>MLDSKLKAPVFTVRTQGREYGEFVLEPLERGFGVTLGNPLRRILLSSIPGTAVTSVYIEDVLHEFSTIPGVKEDVVEIILNLKELVVRFLNPSLQTVTLLLKAEGPKEVKARDFLPVADVEIMNPDLHIATLEEGGRLNMEVRVDRGVGYVPAEKHGIKDRINAIPVDAVFSPVRRVAFQVEDTRLGQRTDLDKLTLRIWTDGSVTPLEALNQAVEILREHLTYFSNPQAAAVAAPEEAKEPEAPPEQEEELDLPLEELGLSTRVLHSLKEEGIESVRALLALNLKDLKNIPGIGERSLEEIKEALEKKGFTLKE[2x];> MEIKRFGRIREVIPLPPLTEIQVESYRRALQADVPPEKRENVGIQAAFRETFPIEEEDKGKGGLVLDFLEYRLGEPPFPQDECREKDLTYQAPLYARLQLIHKDTGLIKEDEVFLGHIPLMTEDGSFIINGADRVIVSQIHRSPGVYFTPDPARPGRYIASIIPLPKRGPWIDLEVEPNGVVSMKVNKRKFPLVLLLRVLGYDQETLARELGAYGELVQGLMDESVFAMRPEEALIRLFTLLRPGDPPKRDKAVAYVYGLIADPRRYDLGEAGRYKAEEKLGIRLSGRTLARFEDGEFKDEVFLPTLRYLFALTAGVPGHEVDDIDHLGNRRIRTVGELMTDQFRVGLARLARGVRERMLMGSEDSLTPAKLVNSRPLEAAIREFFSRSQLSQFKDETNPLSSLRHKRRISALGPGGLTRERAGFDVRDVHRTHYGRICPVETPEGANIGLITSLAAYARVDELGFIRTPYRRVVGGVVTDEVVYMTATEEDRYTIAQANTPLEGNRIAAERVVARRKGEPVIVSPEEVEFMDVSPKQVFSVNTNLIPFLEHDDANRALMGSNMQTQAVPLIRAQAPVVMTGLEERVVRDSLAALYAEEDGEVAKVDGNRIVVRYEDGRLVEYPLRRFYRSNQGTALDQRPRVVVGQRVRKGDLLADGPASENGFLALGQNVLVAIMPFDGYNFEDAIVISEELLKRDFYTSIHIERYEIEARDTKLGPERITRDIPHLSEAALRDLDEEGVVRIGAEVKPGDILVGRTSFKGESEPTPEERLLRSIFGEKARDVKDTSLRVPPGEGGIVVRTVRLRRGDPGVELKPGVREVVRVYVAQKRKLQVGDKLANRHGNKGVVAKILPVEDMPHLPDGTPVDVILNPLGVPSRMNLGQILETHLGLAGYFLGQRYISPIFDGAKEPEIKELLAQAFEVYFGKRKGEGFGVDKREVEVLRRAEKLGLVTPGKTPEEQLKELFLQGKVVLYDGRTGEPIEGPIVVGQMFIMKLYHMVEDKMHARSTGPYSLITQQPLGGKAQFGGQRFGEMEVWALEAYGAAHTLQEMLTLKSDDIEGRNAAYEAIIKGEDVPEPSVPESFRVLVKELQALALDVQTLDEKDNPVDIFEGLASKR;> MKKEVRKVRIALASPEKIRSWSYGEVEKPETINYRTLKPERDGLFDERIFGPIKDYECACGKYKRQRFEGKVCERCGVEVTKSIVRRYRMGHIELATPAAHIWFVKDVPSKIGTLLDLSATELEQVLYFSKYIVLDPKGAILNGVPVEKRQLLTDEEYRELRYGKQETYPLPPGVDALVKDGEEVVKGQELAPGVVSRLDGVALYRFPRRVRVEYVKKERAGLRLPLAAWVEKEAYKPGEILAELPEPYLFRAEEEGVVELKELEEGAFLVLRREDEPVATYFLPVGMTPLVVHGEIVEKGQPLAEAKGLLRMPRQVRAAQVEAEEEGETVYLTLFLEWTEPKDYRVQPHMNVVVPEGARVEAGDKIVAAIDPEEEVIAEAEGVVHLHEPASILVVKARVYPFEDDVEVSTGDRVAPGDVLADGGKVKSDVYGRVEVDLVRNVVRVVESYDIDARMGAEAIQQLLKELDLEALEKELLEEMKHPSRARRAKARKRLEVVRAFLDSGNRPEWMILEAVPVLPPDLRPMVQVDGGRFATSDLNDLYRRLINRNNRLKKLLAQGAPEIIIRNEKRMLQEAVDALLDNGRRGAPVTNPGSDRPLRSLTDILSGKQGRFRQNLLGKRVDYSGRSVIVVGPQLKLHQCGLPKRMALELFKPFLLKKMEEKGIAPNVKAARRMLERQRDIKDEVWDALEEVIHGKVVLLNRAPTLHRLGIQAFQPVLVEGQSIQLHPLVCEAFNADFDGDQMAVHVPLSSFAQAEARIQMLSAHNLLSPASGEPLAKPSRDIILGLYYITQVRKEKKGAGLEFATPEEALAAHERGEVALNAPIKVAGRETSVGRLKYVFANPDEALLAVAHGIVDLQDVVTVRYMGKRLETSPGRILFARIVAEAVEDEKVAWELIQLDVPQEKNSLKDLVYQAFLRLGMEKTARLLDALKYYGFTFSTTSGITIGIDDAVIPEEKKQYLEEADRKLLQIEQAYEMGFLTDRERYDQILQLWTETTEKVTQAVFKNFEENYPFNPLYVMAQSGARGNPQQIRQLCGLRGLMQKPSGETFEVPVRSSFREGLTVLEYFISSHGARKGGADTALRTADSGYLTRKLVDVTHEIVVREADCGTTNYISVPLFQPDEVTRSLRLRKRADIEAGLYGRVLAREVEVLGVRLEEGRYLSMDDVHLLIKAAEAGEIQEVPVRSPLTCQTRYGVCQKCYGYDLSMARPVSIGEAVGIVAAQSIGEPGTQLTMRTFHTGGVAGAADITQGLPRVIELFEARRPKAKAVISEIDGVVRIEETEEKLSVFVESEGFSKEYKLPKEARLLVKDGDYVEAGQPLTRGAIDPHQLLEAKGPEAVERYLVEEIQKVYRAQGVKLHDKHIEIVVRQMMKYVEVTDPGDSRLLEGQVLEKWDVEALNERLIAEGKTPVAWKPLLMGVTKSALSTKSWLSAASFQNTTHVLTEAAIAGKKDELIGLKENVILGRLIPAGTGSDFVRFTQVVDQKTLKAIEEARKEAVEAKERPAARRGVKREQPGKQA;> MAEPGIDKLFGMVDSKYRLTVVVAKRAQQLLRHGFKNTVLEPEERPKMQTLEGLFDDPNAVTWAMKELLTGRLVFGENLVPEDRLQKEMERLYPVEREE;> MEIALERIYGHRLALPQVGAALLFAQEAPPALLLVPEARLRRYRDLSAFGAKVYVNPGLEALEEKALFVLSYEEALSPFPEDPEAWRLLLEVGRAYPREALLSRLLKLGYARDEDYRVLGEVVELGEVRLEFFGDELERLVVRGEERRRHVLLPKPGKAEGFTSKKVLHFPGPVYLDTPALAPKALWPLLAGRPWVALGGGVELPPLELGARPLPPYRGSLKALEKDLARWLAEGKRVHLFVGHARTLEYLKRRLQAFSPLILDRFPGPKGRLALLPGDFEGGAEWGEWVLLTEALVFATGGVRARVRVGEGLSDPGALSPGDYLIHPEHGVGQYLGLETREVLGVKRDYLVLRYKGEGKLYLPVEQLPLLKRHPGTTDDPPELSSLGKNEWQRAKEKARKDVEELAGRLLVLQAKRKATPGRAFPPLPEWDPLVEKGFPYELTPDQKRALEEVLRDLESPHPMDRLVSGDVGFGKTEVALRAAHRVVGHGAQVAFLVPTTLLAEQHGKTFRERFQGLPVRVAVLSRFTPPKEEEAILKGLAEGTVDIVIGTHRLLQEDVRFRDLGLLIVDEEHRFGVAQKERIRELKAEVDTLYLSATPIPRTLYSALVGLKDLSSIQTPPPGRKPIKTFLAPFDPLLVREAILFELERGGKVFYVHDRVASIEARRRFLESLVPEARIGVVHGQMPESLIEETMLLFAEGAYDVLLATTIIEAGLDVPEANTILIERADRLGLATLYQLRGRVGRREEEAYAYLFHPPRLTEAAEKRLAAIADLSDLGSGHLLAERDMEIRGVGNLLGPEQHGHIRALSLEVYTELLEEAIRKLKGEVKEERRHVTLDLALSARLPAEYVGSLEARSRYYSRFAEAKSLAELSRLVRELKERYGPLPEEAENFVALARLRLVAERKGVVSITEGLTHLEVVFPRYPLDYDARGLKGLPYRVELTQYPPGFRLEKKGLRPRDYPEALMEVLYLFADL

Mfd is a highly conserved ATP-dependent DNA translocase in bacteria. It recognizes stalled RNA polymerase (RNAP) and removes it from DNA, leading to Mfd-dependent transcription termination. Mfd can be functionally dissected into an N-terminal region (NTR), an RNAP interacting domain (RID), a translocation module (TM), and a C-terminal domain (CTD). Here, we report the single-particle cryo-electron microscopy structures of T. thermophilus Mfd-RNAP complex with and without ATPγS.

The cryo-EM structures of MTC with and without ATPγS (MTCATPγS and MTCapo) were determined at 4.1 and 5.0 Å, respectively. The conformations of RNAP in both structures are similar with a root-mean-square deviation (RMSD) of 0.85 Å (2954 Cαs aligned). The interactions between Mfd and RNAP are essentially the same in MTC with and without ATPγS. There is a kink of 29° in MTCATPγS and 36° in MTCapo at position –16, which is consistent with the single molecule observation. Compared with the cryo-EM structure of Mfd in the absence of RNAP, the RH rotates ∼45° and the RID translates ∼70 Å in MTCATPγS and MTCapo, indicating that RNAP induces domain repositioning. The TM first binds DNA in an open conformation. Compared to MTCapo, TD2 rotates by ∼33° toward TD1 in MTCATPγS. Superposition of TD1 with and without ATPγS results in different registers of TD2, which are offset along the DNA by ∼1 bp in the direction of translocation, suggesting that the step size of Mfd is 1 bp. Finally, ATP hydrolysis and ADP dissociation reset Mfd in an open conformation at the new DNA register. On the contrary, the clamp is open in MTC structures.> SSQRSVARMDGDVIIGALFSVHHQPPAEKVPERKCGEIREQYGIQRVEAMFHTLDKINADPVLLPNITLGSEIRDSCWHSSVALEQSIEFIRDSLISIRDEKDGLNRCLPDGQTLPPGRTKKPIAGVIGPGSSSVAIQVQNLLQLFDIPQIAYSATSIDLSDKTLYKYFLRVVPSDTLQARAMLDIVKRYNWTYVSAVHTEGNYGESGMDAFKELAAQEGLCIAHSDKIYS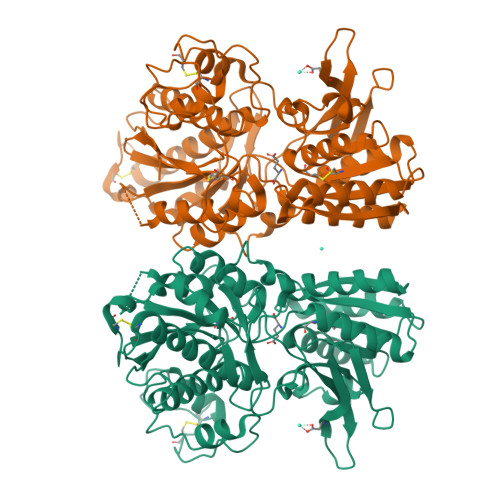NAGEKSFDRLLRKLRERLPKARVVVCFCEGMTVRGLLSAMRRLGVVGEFSLIGSDGWADRDEVIEGYEVEANGGITIKLQSPEVRSFDDYFLKLRLDTNTRNPWFPEFWQHRFQCRLPGHLLENPNFKKVCTGNESLEENYVQDSKMGFVINAIYAMAHGLQNMHHALCPGHVGLCDAMKPIDGRKLLDFLIKSSFVGVSGEEVWFDEKGDAPGRYDIMNLQYTEANRYDYVHVGTWHEGVLNIDDYKIQMNKSGMVRS Multiple antibiotic-resistance regulator (MarR) family proteins are dimeric transcription factors. Binding of effector molecules to MarR proteins gives rise to conformational changes of the MarR homodimer, which sequentially result in dissociation of the repressor from DNA and induction of gene expression. The draft genome sequence of the psychrophilic bacterium Paenisporosarcina sp. strain TG-14, which was isolated from sediment-laden basal ice (Taylor glacier, McMurdo dry valley) in Antarctica, has previously been reported and a gene encoding a MarR family protein has been discovered in the genome information. The crystal structure of PaMarR exhibits an overall architecture comprising a dimerization domain and a DNA-binding domain containing a winged helix–turn–helix motif, which is commonly observed in MarR family proteins.

The structure of PaMarR in complex with palmitic acid has been determined at 1.6 Å resolution. The crystal structure of PaMarR belonged to space group P41212 and contained one molecule in the asymmetric unit. Specifically, the side chains of Val15, Val23, Trp32, Leu111, Ile115, Met119, Val123, Ile128, Phe131, Phe135, Leu138 and Leu142 in chain A, and Ile5, Ala8, Val9 and Phe12 in chain B, form a hydrophobic cavity. The carbon chain moiety of palmitic acid interacts with hydrophobic residues, such as Val15, Val23, Trp32, Leu111, Val123 and Phe131 in chain A and Ile5, Ala8 and Phe12 in chain B [Fig. 2(d)], and the carboxyl acid group of palmitic acid interacts with the side chain of Glu13 located on the α1 helix from the other subunit [Fig. 2(e)]. The palmitic acid molecule was probably derived from the LB medium used during cell culture and protein production; palmitic acid was not supplied in the crystallization step. Accordingly, the B-factor distribution among PaMarR, BsMarR and StMarR was analysed. As shown in Fig. 4(e), the DNA-binding domain of PaMarR exhibits relatively high B-factor values, with a disordered region between the β1 and β2 strands. The conformation observed in the PaMarR structure seems to render the effector-binding site narrower, creating an effector-fitted structure.

> MDKRIQEAVSLFEEVLIYGTERVIRSVDDPLWREYSPEQMQVLKLIYKEGEITSGRLAILQGVHKSAISNRLKKLIEKEVISIKPSGDKREKILVLTALGETVIKQSDAVLHEYIGKLMTNKVDDQEIEQFLVTFRKLKEILKMNGV> VTPEQLATLSHEFRTPLNGVLGMARLLENTKLTAEQRSYVTALRESGDHLLSLVNDVLHFARLGAAAIELSLAPVDIEGLLRQVAELMSPRAHEKGIEIAWAVSSPLPTILADEGRLRQILLNFAGNAVKFTEAGGVLLTASAIDGGRVRFSVADTGPGVA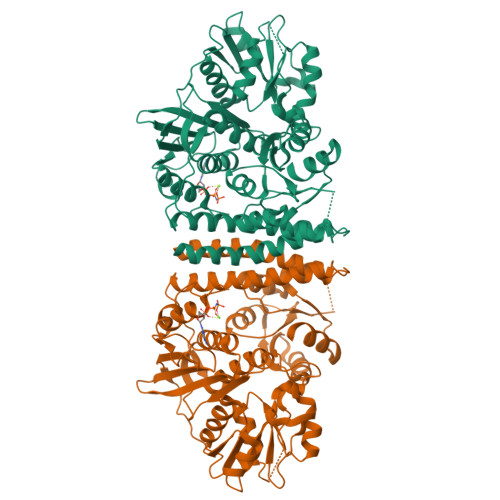PDARARIFEAFVQTDVTHATQLGGAGLGLAIVSRLSAAMGGAVGVGGELGQGAEFWFEAPFATAAAPLRAAPLEGRNVAIASPNAIVRAATARQIEAAGGRAYAAVDIASALAGAPADAVLLIDAALSGPRGALKPPAGRRSVVLLTPEQRDRIDRLKAAGFSGYLIKPLRAASLVAQVLQAVTADGVAEDEPAHDDRIAGAVASGARVLLAEDNPINALLARTLLEREGCIVDRVADGEQAIAAASAGVYDLILMDLRMPGLTGIEAARALRAKGVATPIAALTADAFDEDRRTCLAAGMDDFLVKPLTQEALRDALKRWTT>PISPIETVPVKLKPGMDGPKVKQWPLTEEKIKALVEICTEMEKEGKISKIGPENPYNTPVFAIKKKDSTKWRKLVDFRELNKRTQDFWEVQLGIPHPAGLKKKKSVTVLDVGDAYFSVPLDEDFRKYTAFTIPSINNETPGIRYQYNVLPQGWKGSPAIFQSSMTKILEPFKKQNPDIVIYQYMDDLYVGSDLEIGQHRTKIEELRQHLLRWGLTTPDKKHQKEPPFLWMGYELHPDKWTVQPIVLPEKDSWTVNDIQKLVGKLNWASQIYPGIKVRQLCKLLRGTKALTEVIPLTEEAELELAENREILKEPVHGVYYDPSKDLIAEIQKQGQGQWTYQIYQEPFKNLKTGKYARMRGAHTNDVKQLTEAVQKITTESIVIWGKTPKFKLPIQKETWETWWTEYWQATWIPEWEFVNTPPLVKLWYQLEKEPIVGAETFYVDGAANRETKLGKAGYVTNKGRQKVVPLTNTTNQKTQLQAIYLALQDSGLEVNIVTDSQYALGIIQAQPDKSESELVNQIIEQLIKKEKVYLAWVPAHKGIGGNEQVDKLVSAGIRKIL[2x];>[2x]PISPIETVPVKLKPGMDGPKVKQWPLTEEKIKALVEICTEMEKEGKISKIGPENPYNTPVFAIKKKDSTKWRKLVDFRELNKRTQDFWEVQLGIPHPAGLKKKKSVTVLDVGDAYFSVPLDEDFRKYTAFTIPSINNETPGIRYQYNVLPQGWKGSPAIFQSSMTKILEPFKKQNPDIVIYQYMDDLYVGSDLEIGQHRTKIEELRQHLLRWGLTTPDKKHQKEPPFLWMGYELHPDKWTVQPIVLPEKDSWTVNDIQKLVGK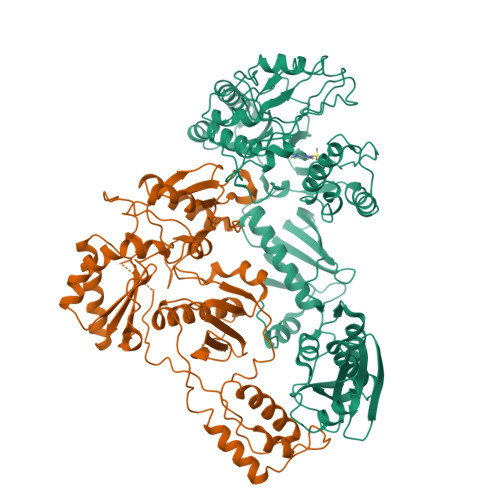LNWASQIYPGIKVRQLCKLLRGTKALTEVIPLTEEAELELAENREILKEPVHGVYYDPSKDLIAEIQKQGQGQWTYQIYQEPFKNLKTGKYARMRGAHTNDVKQLTEAVQKITTESIVIWGKTPKFKLPIQKETWETWWTEYWQATWIPEWEFVNTPPLVKLWY>[3x]EKIKICLQKQVNSSFSLHNGFGGNLYATEEKRMFELVKPKAGASVLNQSTWIGFGDSRTDKSNSAFPRSADVSAKTADKFRFLSGGSLMLSMFGPPGKVDYLYQGCGKHKVFYEGVNWSPHAAINCYRKNWTDIKLNFQKNIYELASQSHCMSLVNALDKTIPLQVTAGTAGNCNNSFLKNPALYTQEVKPSENKCGKENLAFFTLPTQFGTYECKLHLVASCYFIYDSKEVYNKRGCDNYFQVIYDSFGKVVGGLDNRVSPYTGNSGDTPTMQCDMLQLKPGRYSVRSSPRFLLMPERSYCFDMKEKGPVTAVQSIWGKGRESDYAVDQACLSTPGCMLIQKQKPYIGEADDHHGDQEMRELLSGLDYEARCISQSGWVNETSPFTEKYLLPPKFGRCPLAAKEESIPKIPDGLLIPTSGTDTTVTKPKSR;>[3x]IFGIDD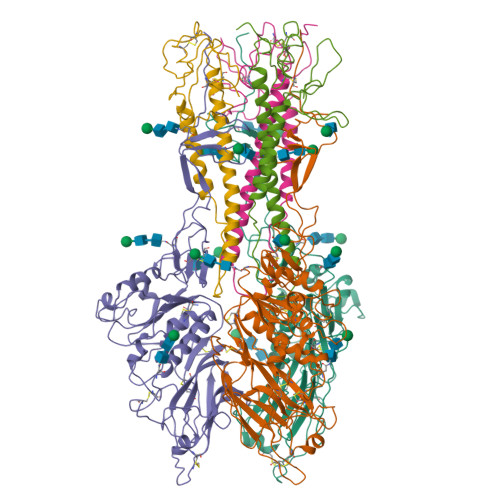LIIGVLFVAIVETGIGGYLLGSRKESGGGVTKESAEKGFEKIGNDIQILKSSINIAIEKLNDRISHDEQAIRDLTLEIENARSEALLGELGIIRALLVGNISIGLQESLWELASEITNRAGDLAVEVSPGCWIIDNNICDQSCQNFIFKFNETAPVPTIPPLDTKIDLQ>[2x]MGRGKRRAKTRNIAIASTKEVQWQGIFMIIVWLCVMGSLIFFANPEASRRVFAKFSHLQSFYGATSVAFAFATGLDILAYVNAVSDEKRVLSGILAYVDGVACISYLSMATLNLYFLVDSTQGNPVWLMRYAEWIITCPTLLYWCGLASRADRSSVSDIATADALLLAGGALSSILPSWPAFFVFAGSFATYIYVMLHMWGMFGKAMQPDF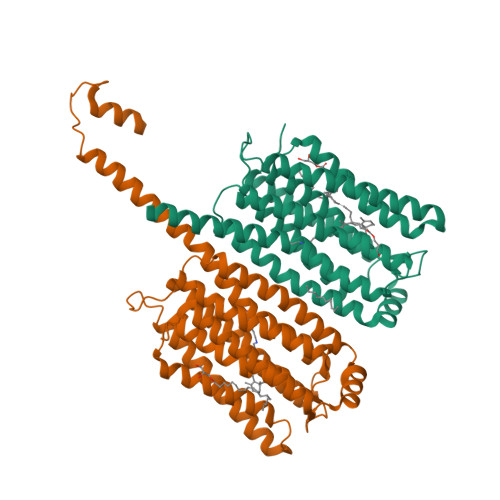QPPPPLPRHALHLLRCEIVMSWSIFPLVEFLRRQGYIDFQVGEAMNCVADYAAKVGLAMIMVNCNLEQINALRVQQMHSALTGMLKVMRKTNLSSSRMAQLDGVDDDVKSWIMNEFSGSTDGKGGDDAKAQQRARGENLYFQ6,7,8,9-TETRAHYDROXY-5-METHYLCARBOXAMIDO-2-OXONONANOIC ACID | C11 H19 N O8 | 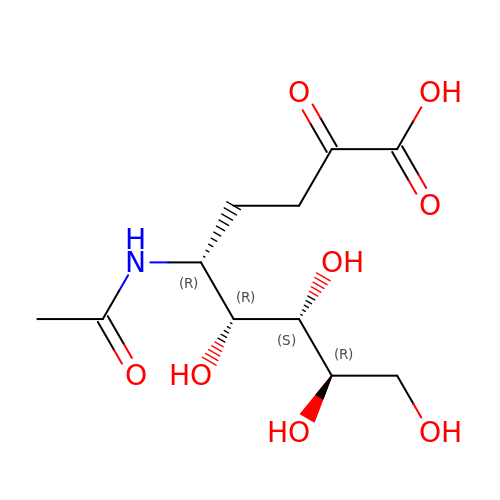HWTGNSKUIIUDOU-PEBGCTIMSA-N SNARE (soluble N-ethylmaleimide-sensitive factor (NSF) attachment protein receptor) proteins drive membrane fusion at different cell compartments as their core domains zipper into a parallel four-helix bundle. After fusion, these bundles are disassembled by the AAA+ (ATPase associated with diverse cellular activities) protein Sec18/NSF and its adaptor Sec17/α-SNAP to make them available for subsequent rounds of membrane fusion. The disassembly requires multiple ATP hydrolysis events in the presence of Mg2+; as few as six ATP hydrolysis events are sufficient. The side-loading and side-release mechanism explains how Sec18/NSF can disassemble SNAREs with constrained topologies.

We chose the Sso1–Sec9–Snc1/Snc2 complex (referred to as the ySNARE complex) because each component of this complex crosslinked with high confidence to the D2 domain of Sec18 (Snc1 is highly homologous to Snc2). We prepared the y20S complex in a nonhydrolyzing condition and, after single-particle cryo-EM data collection and processing, we obtained 381,591 high-quality particles that yielded eight three-dimensional (3D) classes into which models were built. In the structures of all eight classes, Sso1 is threaded through the D1 pore of Sec18. A characteristic phenylalanine side-chain density in Sso1 is present at the same position relative to Sec18 in all classes, allowing for reliable indexing of Sso1. The nucleotide states and the arrangements of D1 around the substrate were also the same among all eight classes, with the ADP-engaged E protomer forming the top of a spiral staircase of tyrosine residues. Protomers D, B and C were all ATP bound and formed the middle of the staircase. The bottom protomer, A, formed the base of the staircase. Protomer F, with no apparent density for nucleotide in D1, was not associated with Sso1. Given that this charge distribution is replicated between each pair of D2 subdomains around the D2 surface, it is unsurprising that the Habc domain adopts multiple corresponding rotational states over the eight classes, presumably because of the flexible linker that follows it.

>[6x]GAHMFKIPGFGKAAANHTPPDMTNMDTRTRHLKVSNCPNNSYALANVAAVSPNDFPNNIYIIIDNLFVFTTRHSNDIPPGTIGFNGNQRTWGGWSLNQDVQAKAFDLFKYSGKQSYLGSIDIDISFRARGKAVSTVFDQDELAKQFVRCYESQIFSPTQYLIMEFQGHFFDLKIRNVQAIDLGDIEPTSAVATGIETKGILTKQTQINFFKGRDGLVNLKSSNSLRPRSNAVIRPDFKFEDLGVGGLDKEFTKIFRRAFASRIFPPSVIEKLGISHVKGLLLYGPPGTGKTLIARKIGTMLNAKEPKIVNGPEILSKYVGSSEENIRNLFKDAEAEYRAKGEESSLHIIIFDELDSVFKQRGSRGDGTGVGDNVVNQLLAKMDGVDQLNNILVIGMTNRKDLIDSALLRPGRFEVQVEIHLPDEKGRLQIFDIQTKKMRENNMMSDDVNLAELAALTKNFSGAEIEGLVKSASSFAINKTVNIGKGATKLNTKDIAKLKVTREDFLNALNDVTPAFGISEEDLKTCVEGGMMLYSERVNSILKNGARYVRQVRESDKSRLVSLLIHGPAGSGKTALAAEIALKSGFPFIRLISPNELSGMSESAKIAYIDNTFRDAYKSPLNILVIDSLETLVDWVPIGPRFSNNILQMLKVALKRKPPQDRRLLIMTTTSAYSVLQQMDILSCFDNEIAVPNMTNLDELNNVMIESNFLDDAGRVKVINELSRSCPNFNVGIKKTLTNIETARHDEDPVNELVELMTQSA;>GMSDPVELLKRAEKKGVPSSGFMKLFSGSDSYKFEEAADLCVQAATIYRLRKELNLAGDSFLKAADYQKKAGNEDEAGNTYVEAYKCFKSGGNSVNAVDSLENAIQIFTHRGQFRRGANFKFELGEILENDLHDYAKAIDCYELAGEWYAQDQSVALSNKCFIKCADLKALDGQYIEASDIYSKLIKSSMGNRLSQWSLKDYFLKKGLCQLAATDAVAAARTLQEGQSEDPNFADSRESNFLKSLIDAVNEGDSEQLSEHCKEFDNFMRLDKWKITILNKIKESIQQQEDDLL[3x];> GASHMSSSTPFDPYALSEHDEERPQNVQSKSRTAELQAEIDDTVGIMRDNINKVAERGERLTSIEDKADNLAVSAQGFKRGANRVRKAMWYKDLKMK;> GASHMSYNNPYQLETPFEESYELDEGSSAIGAEGHDFVGFMNKISQINRDLDKYDHTINQVDSLHKRLLTEVNEEQASHLRHSLDNFVAQATDLQFKLKNEIKSAQRDGIHDTNKQAQAENSRQRFLKLIQDYRIVDSNYKEENKEQAKRQYMIIQPEATEDEVEAAISDVGGQQIFSQALLNANRRGEAKTALAEVQARHQELLKLEKSMAELTQLFNDMEELVIEQQENVDVIDKNVEDAQLDVEQGVGHTDKAVKSARKARKNKIR;> GASHIKFTKQSSVASTRNTLKMAQDAERAGMNTLGMLGHQSEQLNNVEGNLDLMKVQNKVADEKVAELKKLNRSILAVHVSNPFNSKRRRREREEQLKNRKIEEKLMREQTSQQLSQSTQRIEGAMNANNNISEVRERYQRKNVLEKAKRYQFENDEEDDEMELEIDRNLDQIQQVSNRLKKMALTTGKELDSQQKRLNNIEESTDDLDINLHMNTNRLAGI> KSKAHKAIELQMALQGLAQSAYKTEDWTLQDTCEELWNTEPTHCFKKGGQTVQVYFDGNKDNCMTYVAWDSVYYMTDAGTWDKTATCVSHRGLYYVK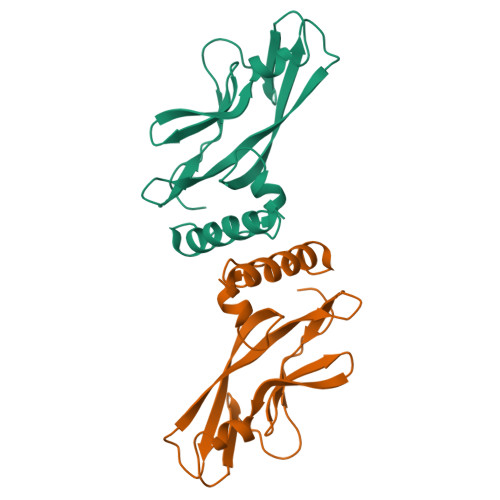EGYNTFYIEFKSECEKYGNTGTWEVHFGNNVIDCNDSMCSTSDDTVS>MAEQVLPQALYLSNMRKAVKIRERTPEDIFKPTNGIIHHFKTMHRYTLEMFRTCQFCPQFREIIHKALIDRNIQATLESQKKLNWCREVRKLVALKTNGDGNCLMHATSQYMWGVQDTDLVLRKALFSTLKETDTRNFKFRWQLESLKSQEFVETGLCYDTRNWNDEWDNLIKMASTDTPMARSGLQYNSLEEIHIFVLCNILRRPIIVISDKMLRSLESGSNFAPLKVGGIYLPLHWPAQECYRYPIVLGYDSHHFVPLVTLKDSGPEIRAVPLVNRDRGRFEDLKVHFLTDPENEMKEKLLKEYLMVIEIPVQGWDHGTTHLNNAAKLDEANLP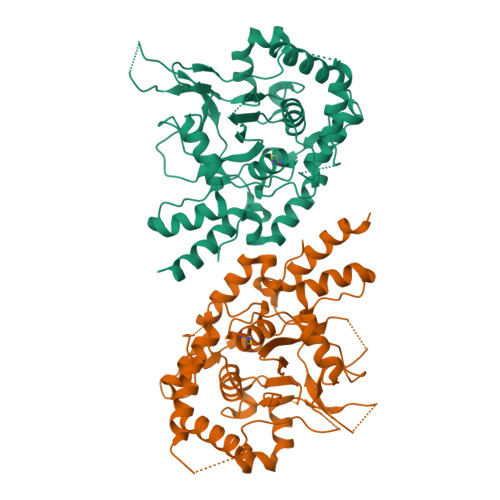KEINLVDDYFELVQHEYKKWQENSEQGRRE[6x]>[4x]STTGIIMENVTAFWEEGFGELLEKVQQSNGDRKHSSDENNVSFSHLCLVGNPVLKNINLNIEKGEMLA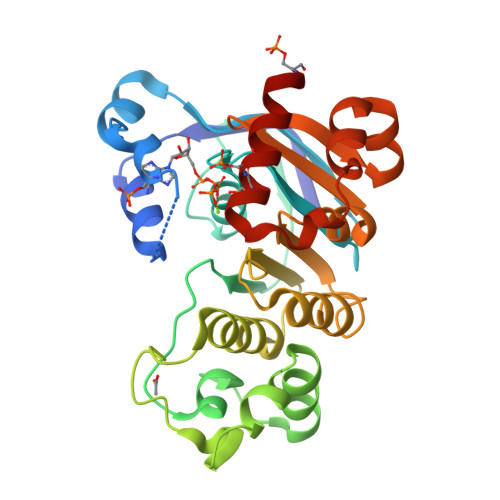ITGSTGSGKTSLLMLILGELEASEGIIKHSGRVSFCSQFSWIMPGTIKENIIFGVSYDEYRYKSVVKACQLQQDITKFAEQDNTVLGEGGVTLSGGQRARISLARAVYKDADLYLLDSPFGYLDVFTEEQVFESCVCKLMANKTRILVTSKMEHLRKADKILILHQGSSYFYGTFSELQSLRPDFSSKLMGYDTFDQFTEERRSSILTETLRRFSVDD>MPHSHLHLDPKVREEARRRLLSAKGHLEGILRMLEDEKVYCVDVLKQLKAVEGALDRVGEMVLRAHLK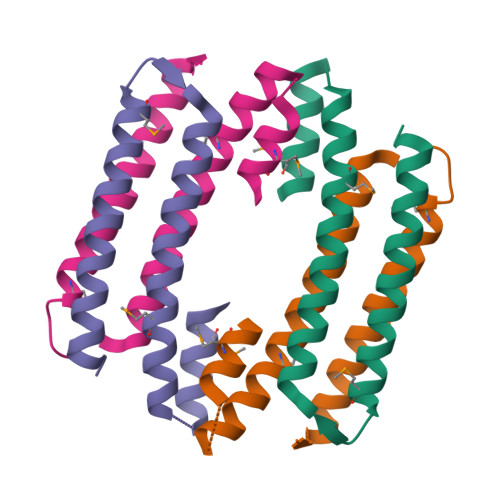DHVATAHERGDVEEIVEELMEALKYR[4x]> GAGNKMGFVVTMLKLIQKK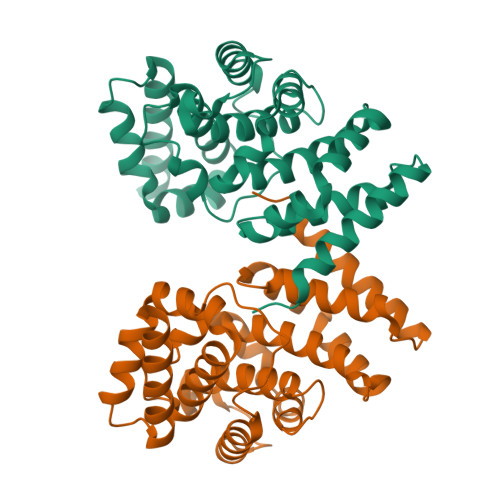LLDKTCDQVMEFSWSALWNITDETPDNCEMFLNFNGMKLFLDCLKEFPEKQELHRNMLGLLGNVAEVKELRPQLMTSQFISVFSNLLESKADGIEVSYNACGVLSHIMFDGPEAWGVCEPQREEVEERMWAAIQSWDINSRRNINYRSFEPILRLLPQGISPVSQHWATWALYNLVSVYPDKYCPLLIKEGGMPLLRDIIKMATARQETKEMARKVIEHCSNFKEENMDTSR> GEPLYENSPEFTPYLETNLGQPTIQSFEQVGTKVNVTVEDERTLVRRNNTFLSLRDVFGKDLIYTLYYWKS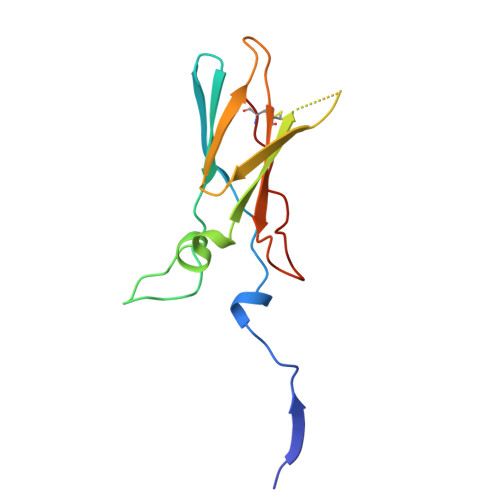SSSGKKTAKTNTNEFLIDVDKGENYCFSVQAVIPSRTVNRKSTDSPVECM> FACKTANGTAIPIGGGSANVYVNLAPVVNVGQNLVVDLSTQIFCHNDYPETITDYVTLQRGSAYGGVLSNFSGTVKYSGSSYPFPTTSETPRVVYNSRTDKPWPVALYLTPVSSAGGVAIKAGSLIAVLILRQTNNANSDDFQFVWNIYANNDVVVPT

E. coli clinical isolates express the FimH adhesin, which consists of a mannose-specific lectin domain connected via a pilin domain to the tip of type 1 pili. The FimH lectin binds specifically to mannose moieties displayed on glycoproteins at the luminal surface of epithelial cells. Mannose binds in a deep and polar pocket at the N-terminal end of FimH, in which the amino acids Phe1, Asn46, Asp47, Asp54, Gln133, Asn135, Asp140 and Phe142 create a dense network of 12 hydrogen bonds with each hydroxyl group of the pyran­ose ring except that at the α-anomeric position of mannose. The interaction of the aglycones with the tyrosine gate formed by two tyrosines (Tyr48 and Tyr137) at the entrance to the FimH binding site contributes significantly to their affinity, for example with a 400-fold increase for HM compared with α-d-manno­pyranoside.

The Y137A mutation, on the other hand, is the most detrimental to FimH affinity and specificity: (i) in the absence of ligand the FimH C-terminal residue Thr158 intrudes into the mannose-binding pocket and (ii) ethylenediaminetetraacetic acid interacts strongly with Glu50, Thr53 and Asn136, in spite of multiple dialysis and purification steps. The ligand-free state of Y137A FimH permits the C-terminal carboxylate of a neighbouring molecule to enter its mannose-binding pocket. The Val155-Val156-Pro157-Thr158 peptide of the FimH lectin domain from an adjacent symmetry-related lectin domain makes a significant intrusion where the oligomannoside glycan is normally bound. In addition, an EDTA buffer molecule is bound in different alternate conformations into a cavity on the FimH surface. Remarkably, EDTA was only contained in the extraction buffer of FimH extraction from the E. coli periplasm, but remained bound during purification and dialysis steps, which did not contain EDTA (see also §2). The EDTA binding site is very close to the mannose-binding pocket and the two sites are coupled by residue Ile52. The Ile52-mediated connection might be needed in WT FimH for proper guidance of the ligand to its binding site. Ile52 is also the residue directly linking the protein-intruded mannose-binding site inside the Y137A mutant FimH, with the EDTA binding site formed by Asn136, Thr53 and Glu50 at the protein surface. The Y137A mutant structure allows the binding of a macromolecule other than mannose in the FimH mannose-binding pocket to be observed for the first time and moreover exposes a hitherto undiscovered adjacent binding pocket on the FimH surface. In the ligand-free state of Y137A FimH, several of the binding-site residues (including Asn136, Tyr137 and Tyr48) already sample backbone dihedral angles that are normally only found in wild-type FimH upon binding of the mannose. In the crystals of the Y137A mutant, a breakdown of the binding site with a severe loss of specificity is observed.4-(4-bromanyl-2-oxidanylidene-3~{H}-benzimidazol-1-yl)-~{N}-(3-methoxy-4-methyl-phenyl)piperidine-1-carboxamide | C21 H23 Br N4 O3 | 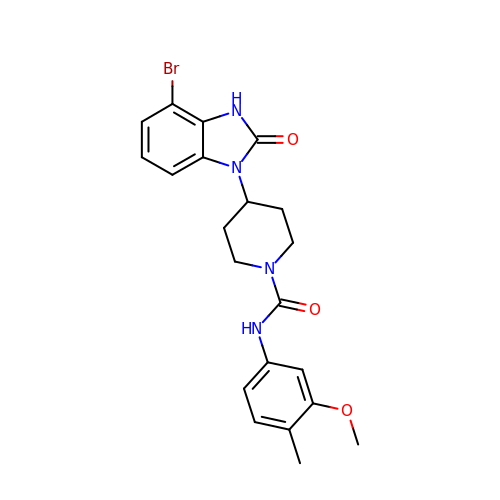JGPXNMHYCZPDRK-UHFFFAOYSA-N>SFKDLNLTDAQKQQIREIMKGQRDQMKRPPLEERRAMHDIIASDTFDKVKAEAQIAKMEEQRKANMLALMETQNKIYNILTPEQKKQFNANFEKRLT[2x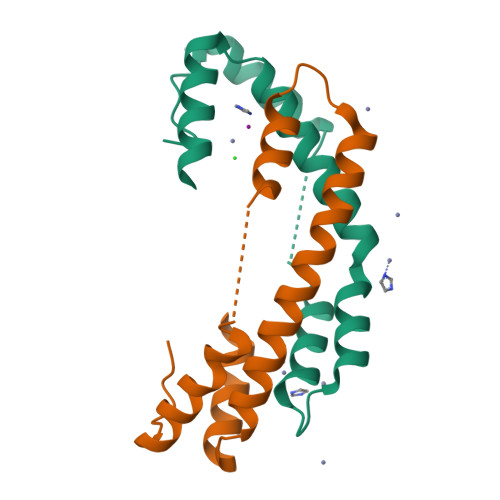]>GSHMASKPVIRVFILTSNNPELRSRLLLFCLRIVLSNGARDSHRFGALLTMFSLPSATMLNHVKLADQSPEADIERVEIDGFEEGSFRLIPNARSGMSRGEINAYAALAEDLPDTLNHATPFVDSEVEGTAWDEIETFLDMCYSVLMQAWIVTCKCMTAPDQPAASIEKRLQKYRQQGRINPRYLLQPEARRIIQNVIRKGMVVRHFLTFELQLARAQSLVSNRYYAMVGDV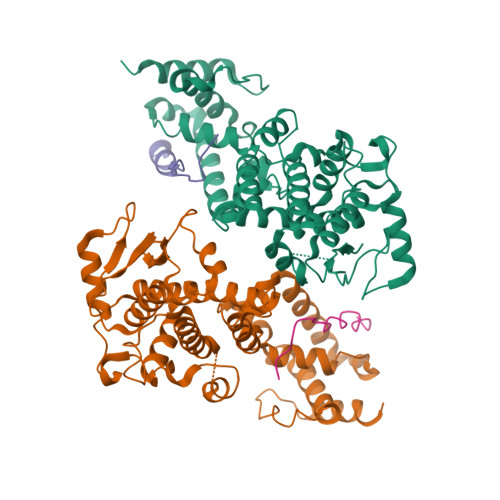GKYIENCGMGGFFLTLKYALGTRWPTLALAAFSGELTKLKSLMALYQTLGEQARYLALLESPHLMDFAAANYPLLYSYAMGIGYVLDVNMRNYAFSRSYMNKTYFQLGMETARKQM[2x];>DPTDLSFSPDEINKLIETGLNTVEYFTSQQVTGTSSLGKNTIPPGVTGL[2x]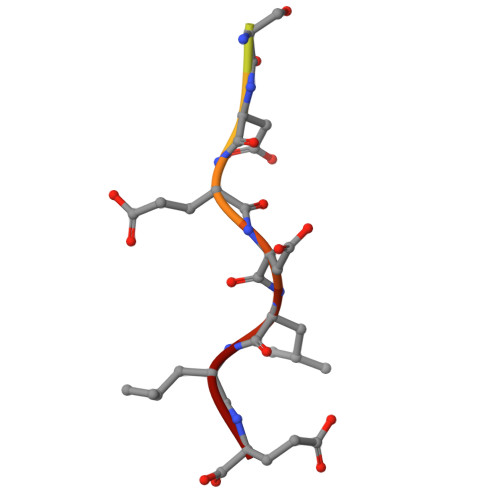> SGYHDDSDEDLLE> MPELAVRTEFDYSSEIYKDAYSRINAIVIEGEQEAYSNYLQMAELLPEDKEELTRLAKMENRHKKGFQACGNNLQVNPDMPYAQEFFAGLHGNFQHAFSEGKVVTCLLIQALIIEAFAIAAYNIYIPVADDFARKITEGVVKDEYTHLNYGEEWLKANFATAKEELEQANKENLPLVWKMLNQVQGDAKVLGMEKEALVEDFMIS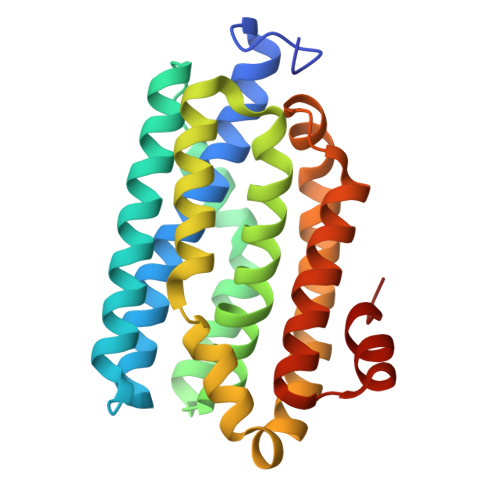YGEALSNIGFSTREIMRMSSYGLAGV dimethyl 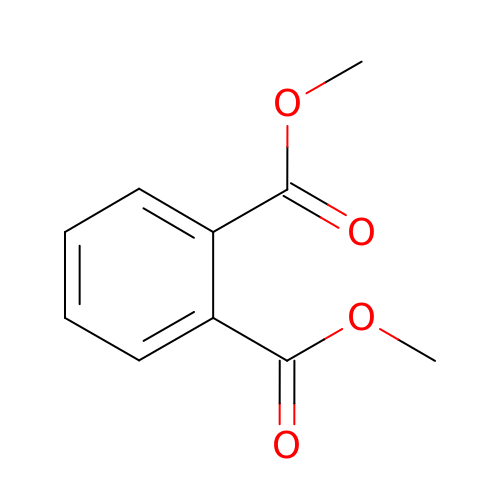benzene-1,2-dicarboxylate | C10 H10 O4 | NIQCNGHVCWTJSM-UHFFFAOYSA-N>[6x]HDCVNI;>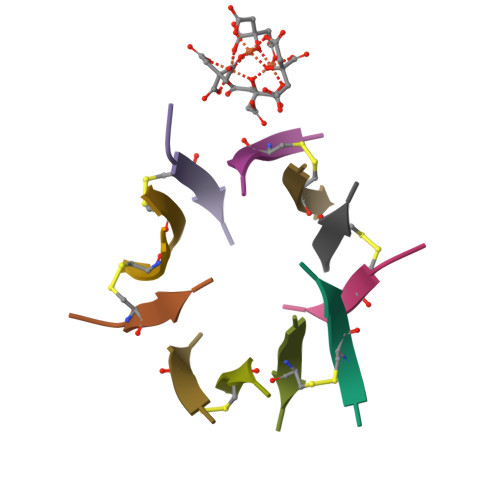[6x]EQMCIT>AVSKVYARSVYDSRGNPTVEVELTTEKGVFRSIVPSGANTGVHEALEMRDGDKSKWMGKGVLHAVKNVNDVIAPAFVKANIDVKDQKAVDDFLISLDGTANKSKLGANAILGVSLAASRAAAAEKNVPLYKHLADLSKSKTSPYVLPVPFLNVLNGGSHAGGALALQEFMIAPTGAKTFAEALRIGSEVYHNLKSLTKKRYGASAGNVGDEGGVAPNIQTAEEALDLIVDAIKAAGHDGKIKIGLDCASSEFFKDGKYDLDFKNPNSDKSKWLTGPQLADLYHSLMKRYPIVSIEDPFAEDDWEAWSHFFKTAGIQIVADRLTVTNPKRIATAIEKKAADALLLKVNQIGTLSESIKAAQDSFAAGWGVMVSHRSGETEDTFIADLVVGLRTGQIKTGAPARSERLAKLNQLLRIEEE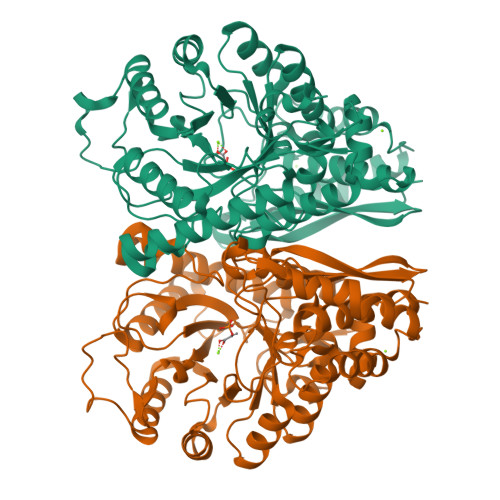LGDNAVFAGENFHHGDKLLHHHHHH[2x]>MSTGDFLTKGIELVQKAIDLDTATQYEEAYTAYYNGLDYLMLALKYEKNPKSKDLIRAKFTEYLNRAEQLKKHLESEEANAAKKSPSAGSGSNGGNKKISQEEGEDNGGEDNKKLRGALSSAILSEKPNVKWEDVAGLEGAKEALKEAVILPVKFPHLFKGNRKPTSGILLYGPPGTGKSYLAKAVATEANSTFFSVSSSDLVSKWMGESEKLVKQLFAMARENKPSIIFIDQVDALTGTRGEGESEASRRIKTELLVQMNGVGNDSQGVLVLGATNIPWQLDSAIRRRFERRIYIPLPDLAARTTMFEINVGDTPCVLTKEDYRTLGAMTEGYSGSDIAVVVKDALMQPIRKIQSATHFKDVSTEDDETRKLTPCSPGDDGAIEMSWTDIEADELKEPDLTIKDFLKAIKSTRPTVNEDDLLKQEQFTRDFGQE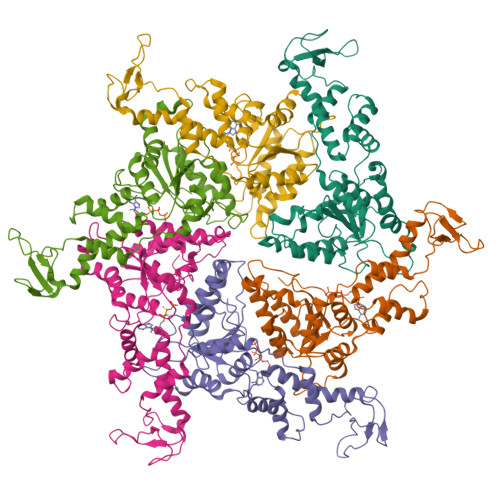GN[6x]>IDVKNAHAVVEQTEENVFLIPLKHLRDSQFVGTLLVGVPPQEIHPIFDTGSTNLWVVTTDCEEESCKKVKRYNPYKSKTFRRSFIGKNLHIVFGSGSISGSIGKETFVLGDHTVRNQTFGLVESESNDSLNGDNIFDYIDFEGIVGLGFPEMLSAGKVSFFDNL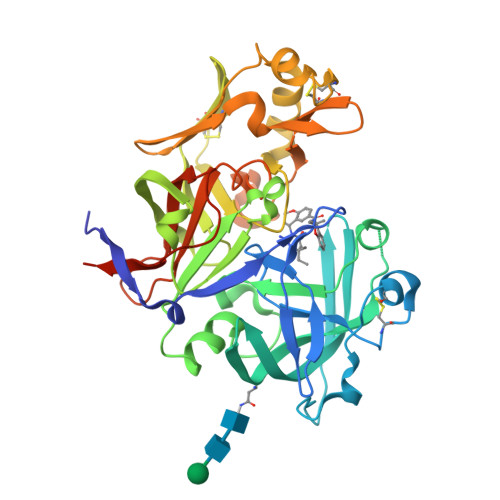LSQNKNLSPQFSFYISPEDNTSTFLVGGVSKSFYEGSIYMLPVVKEYYWEVELDGIYVGEKKICCEEKSYAIFDTGTSYNTMPSAQMKGFFDVVPSAPCTEENYQEVLKNYPVIKYLFGDLVIELLPEEYMILNEESCIPAYMQIDVPSEKNHAYLLGSIAFMRHYYTVFVRGAGGQPSMVGVAKARAAAEAAQKVAELENFYFQGDYKDDDDKH[2x]> GPEIRMDKKSLYKYLLLRSTGDMHKAKSPTIMTRVTNNVY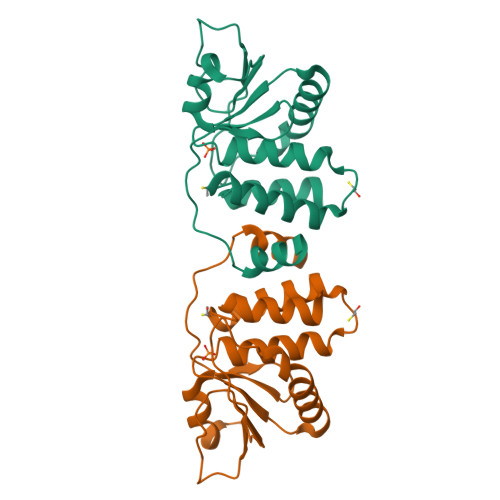LGNYKNAMDAPSSEVKFKYVLNLTMDKYTLPNSNINIIHIPLVDDTTTDISKYFDDVTAFLSKCDQRNEPVLVHSAAGVNRSGAMILAYLMSKNKESLPMLYFLYVYHSMRDLRGAFVENPSFKRQIIEKYVIDKN>[2x]TNATGERNLALIQEVLEVFPETARKERRKHMMVSDPKMKSVGKCIISNRKSQPGVMTVRGCAYAGSKGVVFGPIKDMAHISHGPVGCGQYSRAGRRNYYTGVSGVDSFGTLNFTSDFQERDIVFGGDKKLSKLIEEMELLFPLTKGITIQSECPVGLIGDDISAVANASSKALDKPVIPVRCEGFRGVSQSLGHHIANDVVRDWILNNREGQPFETTPYDVAIIGDYN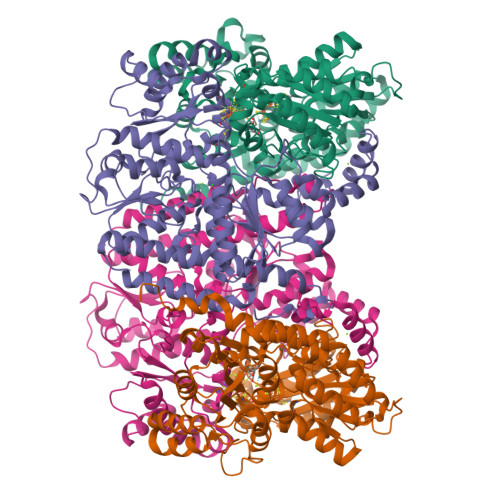IGGDAWASRILLEEMGLRVVAQWSGDGTLVEMENTPFVKLNLVHCYRSMNYIARHMEEKHQIPWMEYNFFGPTKIAESLRKIADQFDDTIRANAEAVIARYEGQMAAIIAKYRPRLEGRKVLLYMGGLRPRHVIGAYEDLGMEIIAAGYEFAHNDDYDRTLPDLKEGTLLFDDASSYELEAFVKALKPDLIGSGIKEKYIFQKMGVPFRQMHSWDYSGPYHGYDGFAIFARDMDMTLNNPAWNELTAPWLKSA;>SQTIDKINSCYPLFEQDEYQELFRNKRQLEEAHDAQRVQEVFAWTTTAEYEALNFRREALTVDPAKACQPLGAVLCSLGFANTLPYVHGSQGCVAYFRTYFNRHFKEPIACVSDSMTEDAAVFGGNNNMNLGLQNASALYKPEIIAVSTTCMAEVIGDDLQAFIANAKKDGFVDSSIAVPHAHTPSFIGSHVTGWDNMFEGFAKTFTADYQGQPGKLPKLNLVTGFETYLGNFRVLKRMMEQMAVPCSLLSDPSEVLDTPADGHYRMYSGGTTQQEMKEAPDAIDTLLLQPWQLLKSKKVVQEMWNQPATEVAIPLGLAATDELLMTVSQLSGKPIADALTLERGRLVDMMLDSHTWLHGKKFGLYGDPDFVMGLTRFLLELGCEPTVILSHNANKRWQKAMNKMLDASPYGRDSEVFINCDLWHFRSLMFTRQPDFMIGNSYGKFIQRDTLAKGKAFEVPLIRLGFPLFDRHHLHRQTTWGYEGAMNIVTTLVNAVLEKLDSDTSQLGKTDYSFDLVR[2x]>MSGNGNAAATAEENSPKMRVIRVGTRKSQLARIQTDSVVATLKASYPGLQFEIIAMSTTGDKILDTALSKIGEKSLFTKELEHALEKNEVDLVVHSLKDLPTVLPPGFTIGAICKRENPHDAVVFHPKFVGKTLETLPEKSVVGTSSLRRAAQLQRKFPHLEFRSIRGNLNTRLRKLDEQQEFSAIILATAGLQRMGWHNRVGQILHPEECMYAVGQGALGVEVRAKDQDILDLVGVLHDPETLLRCIAERAFLRHLEGGCSVPVAVHTAMKDGQL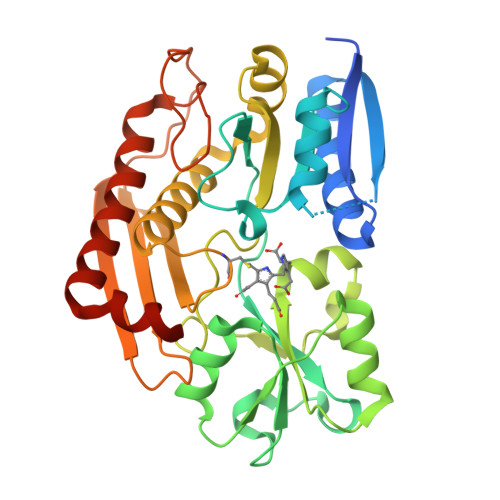YLTGGVWSLDGSDSIQETMQATIHVPAQHEDGPEDDPQLVGITARNIPRGPQLAAQNLGISLANLLLSKGAKNILDVARQLNDAH[2x]> DKRIITDDEIISLSIEFFDQNRLDRKVNKDKEKSKEEVNDKRYLRCPAAMTVMHLRKFLRSKMDIPNTFQIDVMYEEEPLKDYYTLMDIAYIYTWRRNGPLPLKYRVRPTCKRMK

The BMI1 protein, also known as PCGF4 (polycomb group RING finger protein 4), is a central component of the canonical PRC1 complex and has a dual role in PRC1 activity: regulation of H2A ubiquitination activity2627 and mediation of protein–protein interactions. BMI1 is a 37 kDa protein composed of three distinct regions: a N-terminal RING domain2627, a central domain34 and a C-terminal proline-serine rich domain involved in the regulation of protein stability. The central domain of BMI1 was initially predicted as a putative helix-turn-helix (HTH) domain36 and more recently was defined as an ubiquitin-like (UBL) domain, also called RAWUL (RING finger- and WD40-associated ubiquitin-like) domain34. This domain is involved in protein–protein interactions and its best characterized binding partners are the polyhomeotic proteins (PHC1, PHC2, PHC3).

We obtained crystals of BMI1121–235 co-crystalized in the presence of the PHC233–56 fragment, which diffracted to 2.5 Å resolution. The structure confirmed that the central domain of BMI1 adopts an ubiquitin-like (UBL) fold. While we could refine the structure of the UBL domain we were not able to model the PHC2 fragment into the remaining electron density. The unmodelled electron density was found in a wide opening between the β2 strand and α1 helix at the interface between the two BMI1 UBL symmetry related molecules. The incomplete model of the complex is reflected by relatively high R-factor values. Superposition of the PHC2–BMI1 structure with the crystal structure of BMI1 UBL shows that the PHC2 fragment overlaps with the unmodelled electron density observed in the crystal. Since PHC2 binds at the interface of two symmetry related BMI1 UBL molecules, most likely in the crystal structure one molecule of PHC2 is bound to each monomer with 50% occupancy. This unusual binding stoichiometry observed in the crystal structure precludes modelling of the complex solely based on the X-ray data. Analysis of the crystal packing using PISA software suggests two possible homo-oligomerization interfaces. The second interface is centered around Ile212 and involves a cluster of tyrosine side chains (Tyr202, Tyr203, Tyr211 and Tyr213) that form a hydrogen bond network with backbone carbonyls.>[3x]AKTHSVETPYGSVTFTVYGTPAPARPAILTYHDVGLNYKSCFQPLFQFEDMQEIIQNFVRVHVDAPGMEEGAPVFPLGYQYPSLDQLADMIPCVLQYLNFSTIIGVGVGAGAYILARYALNHPDTVEGLVLINIDPNAKGWMDWAAHKLTGLTSSIPEMILGHLFSQEELSGNSELIQKYRNIITHAPNLDNIELYWNSYNNRRDLNFERGGDITLRCP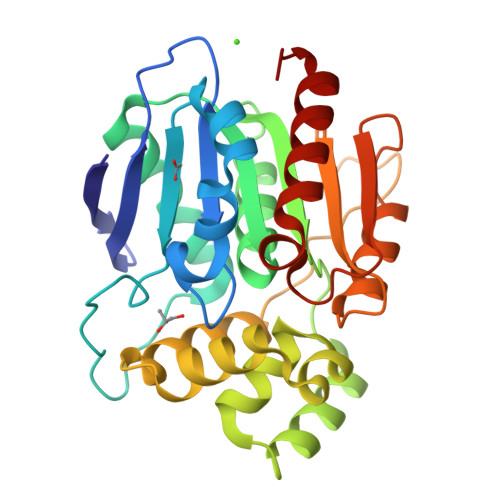VMLVVGDQAPHEDAVVECNSKLDPTQTSFLKMADSGGQPQLTQPGKLTEAFKYFLQGMGYMA>[2x]MLAKDKVALLIGNMNYREHPKLKAPLVDVYELTNLLRQLDFKVVSLLDLTEYEMRNAVDEFLLLLDKGVYGLLYYAGHGYENFGNSFMVPVDAPNPYRSENCLCVQNILKLMQEKETGLNVFLLDMCRKRNDYDDTIPILDALKVTANIVFGYATCQGAEAFEIQHSGLANGIFMKFLKDRLLED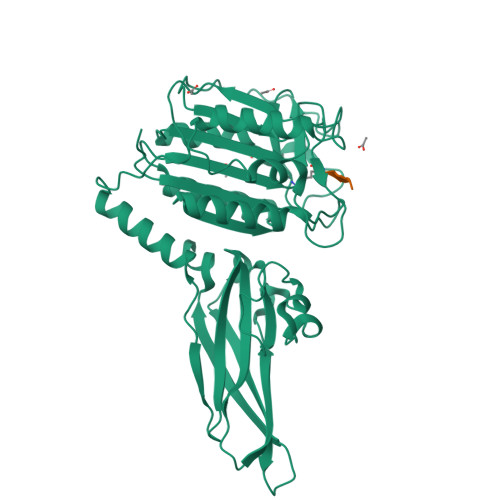KKITVLLDEVAEDMGKCHLTKGKQALEIRSSLSEKRALTDPIQGTEYSAESLVRNLQWAKAHELPESMCLKFDCGVQIQLGFAAEFSNVMIIYTSIVYKPPEIIMCDAYVTDFPLDLDIDPKDANKGTPEETGSYLVSKDLPKHCLYTRLSSLQKLKEHLVFTVCLSYQYSGLEDTVEDKQEVNVGKPLIAKLDMHRHHHHHH;>ALRSX[2x]>SHTENVLDIRTIVANEYAVKTSALEWDVTDIVKNAIIGGISFIPSVGPAISFLVGLFWPQSKENIWEGIVKQIERMIEESALKTIKGILAGDIAYIQERMATVADLLDKHPGSEEARSAFNNLAENIDGYHKKFNNFSDDVNYQILPMFSTTVMMQITYWVAGLERKDEIGLSNIDIEKVRGLIKKTVEQANSYINNIYDRELNDALNNSTADTVANNVMSVHGHCRLHGIEYISIWDRLSEAESVNNRIYVDVLSYSTFFDRQTAKARIQALTPEKDMTPPLKPALNGGKRRKIDSLTGHIVRIGGAARVGGLTVVFDDGSRHQLG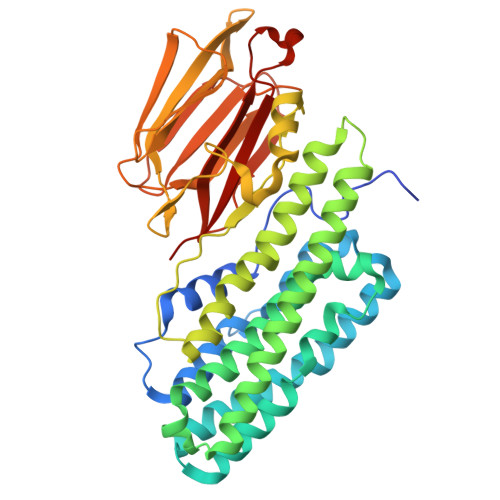TISSETSSISLNGSRITSLEVWGNGAVDQAVFTLRDGRSLSLGSPGTSRYRKFHVGESHYIAGIYLSSDYSPLAGQAANIAVSYQLINDDEK[2x]> MAHHHHHHVDDDDKMKNIGWMLRQRATVSPRLQAYVEPSTDVRMTYAQMNALANRCADVLTALGIAKGDRVALLMPNSVEFCCLFYGAAKLGAVAVPINTRLAAPEVSFILSDSGSKVVIYGAPSAPVIDAIRAQADPPGTVTDWIGADSLAERLRSAAADEPAVECGGDDNLFIMYTSGTTGHPKGVVHTHESVHSAASSWASTIDVRYRDRLLLPLPMFHVAALTTVIFSAMRGVTLIS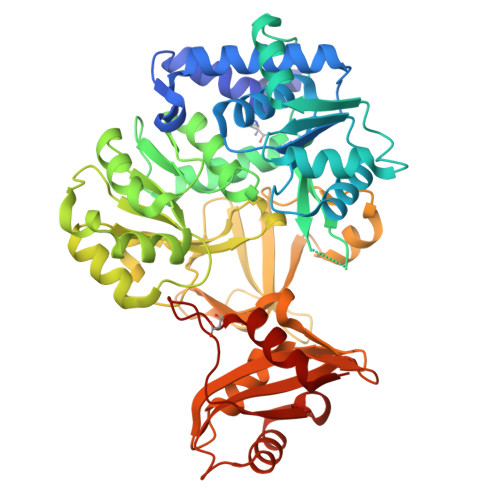MPQFDATKVWSLIVEERVCIGGAVPAILNFMRQVPEFAELDAPDFRYFITGGAPMPEALIKIYAAKNIEVVQGYALTESCGGGTLLLSEDALRKAGSAGRATMFTDVAVRGDDGVIREHGEGEVVIKSDILLKEYWNRPEATRDAFDNGWFRTGDIGEIDDEGYLYIKDRLKDMIISGGENVYPAEIESVIIGVPGVSEVAVIGLPDEKWGEIAAAIVVADQNEVSEQQIVEYCGTRLARYKLPKKVIFAEAIPRNPTGKILKTVLREQYSATVPK1-(3-(5-OXO-4,5-DIHYDRO-1H-1,2,4-TRIAZOL-3-YL)PHENYL)-6-(2'-(PYRROLIDIN-1-YLMETHYL)BIPHENYL-4-YL)-3-(TRIFLUOROMETHYL)-5,6-DIHYDRO-1H-PYRAZOLO[3,4-C]PYRIDIN-7(4H)-ONE | 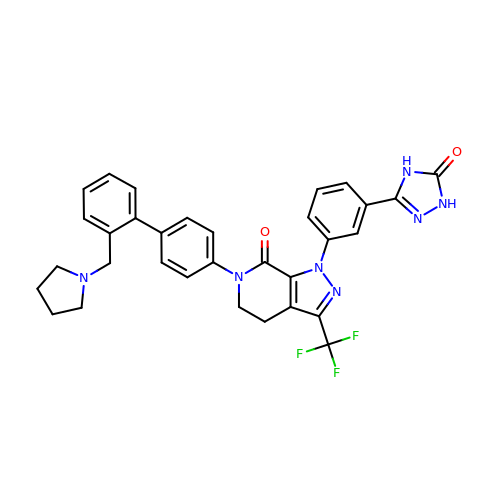C32 H28 F3 N7 O2 | QNPOXJFBWDKXGC-UHFFFAOYSA-N BUTYLPHOSPHONATE | C4 H11 O3 P | 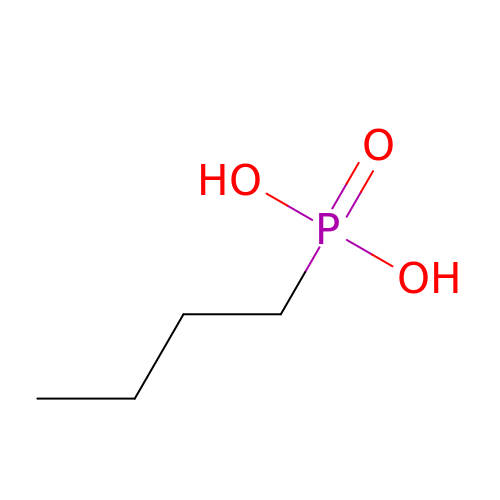UOKRBSXOBUKDGE-UHFFFAOYSA-N>[2x]MGPAFEFAVAMMKRNSSTVKTEYGEFTMLGIYDRWAVLPRHAKPGPTILMNDQEVGVLDAKELVDKDGTNLELTLLKLNRNE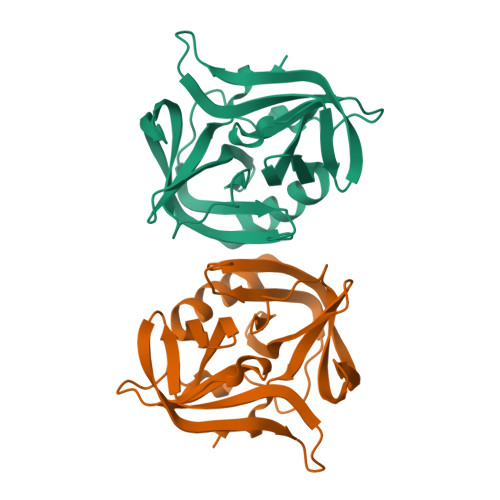KFRDIRGFLAKEEVEVNEAVLAINTSKFPNMYIPVGQVTEYGFLYLGGTPTKRMLMYNFPTRAGQCGGVLMSTGKVLGIHVGGNGHQGFSAALLKHYFNDEQ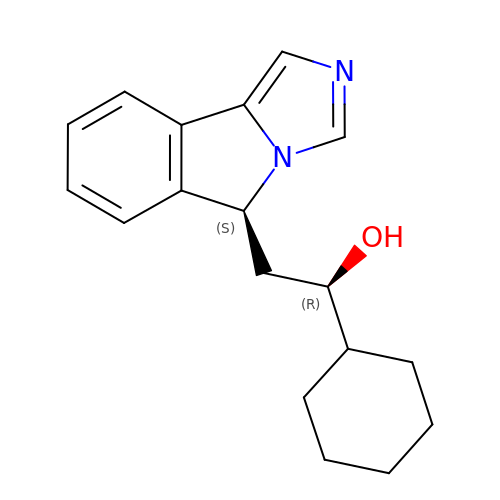(1~{R})-1-cyclohexyl-2-[(5~{S})-5~{H}-imidazo[1,5-b]isoindol-5-yl]ethanol | C18 H22 N2 O | YTRRAUACYORZLX-FUHWJXTLSA-N> MGSDKIHHHHHHMSSAQVNGISKRLIVESPNVKLEDGVLESRFTYRKNHFEHRADGLHVTPKEHDYSFKTVLKPRKTGLLLVGLGGNNGSTAVGSIFANQYAMTWRTKEGHSQANYFGSVTQTATVHLGYDSATQNQIFVPFKDIVPILSPNDLIISGWDISDSNLYEAMGRAKVFEPELQEKLRPFMEPIVPLPSIYYPDFIASNQGDRANNVIPGDNKLEHLEHIRADIRKFKQEHELECVIVLWTANTERYTDVRQGLNATADEIMESIR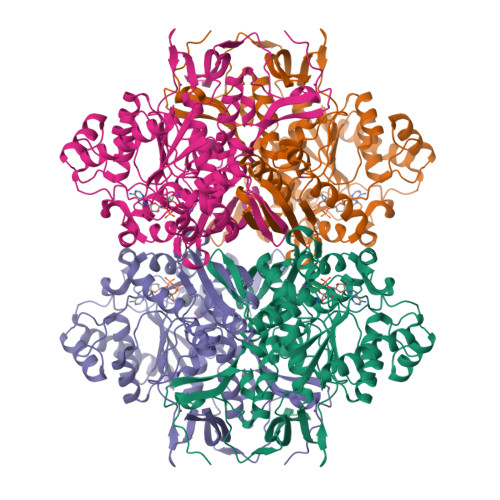VNEDEVSPSNIFAVASILEGAHYINGSPQNTLVPGLIELAERHKVFVGGDDFKSGQTKFKSAFVDFLVSSGMKPESIVSYNHLGNNDGKNLSEARQFRSKEISKSSVVDDMVKSNQILFPDAKNPDYCVVIKYVPYVADSKRAMDEYICSIFMGGKQTFVVHNTCEDSLLASPLIYDLAILTELASRVSYKVDDEYKPFHSVLSILSLLLKAPVVPPGTPISNAFMRQFSTLTKLVTALAGFPSDTDMQIEFFTQLPAAKSKSQ> LKSESAEKTREVLWQQYYASNPPDHAVLEVLATPVREALLARFGQHQGSVVPAIDLPEL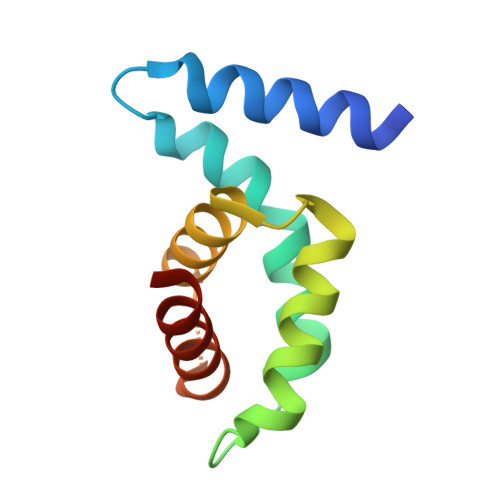RSVLQQFDSFGKRWEAILLQVLEGIKPNESQVGLPYLSELINKELMILLPSNS The core kinase cascade is modulated by adaptor proteins, SAV1 (Salvador, also known as WW45) and MOB1 (encoded by MOB1A and MOB1B in human), both of which work to promote Hippo pathway signaling. MOB1 directly binds to LATS1 and LATS2, and additionally to two related kinases, NDR1, (gene name STK38) and NDR2 (gene name STK38L) via a specialized MOB1-binding domain N-terminal to the kinase domain (15; also see accompanying manuscript by Xiong et al., 2017). Key to its function as a Hippo pathway activator is the ability of MOB1 to bind directly to MST1 and MST2 kinases. We demonstrate that autophosphorylation of MST1 and MST2 on several threonine residues provides multiple MOB1 binding sites with varying binding affinities which in turn contribute to a redundancy of MST1-MOB1 protein interactions in cells.

Peptide overlay analysis (here referred to as Far-Western) revealed that peptides bearing phosphorylated forms of T353 and T367 consistently gave the highest binding signals across the array; nonphosphorylated versions of these peptides generated little to no binding signal. MST1 T353 and T367 peptides displayed high phospho-dependent binding affinities for MOB1A, with Kds of 280 nm and 680 nm for the phosphorylated peptides, respectively, and no detectable binding for the nonphosphorylated peptides. Consistent with their P0 positional binding preferences, human MOB1 bound more tightly to the MST1 pT367 peptide than to the optimized Nud1-like phosphoserine containing peptide than did yeast Mob1, and vice versa. The observed binding modes revealed by these structures are in close agreement with the binding modes reported previously for a yeast Nud1 derived phosphopeptide in complex with human MOB1A, as well as a MST2 T378 phosphopeptide in complex with human MOB1B (see ref 21, 22). As predicted by prior mutational data, the MST1 pT353 and pT367 phosphopeptides bound to the MOB1A phospho-binding pocket first identified by Rock et al., with the phosphate of the P0 threonine directly coordinated by K153, R154 and R157. The p + 1 side chains of M354 and M368 on MST1-pT353 and MST1-pT367 peptides respectively resided in an expansive hydrophobic surface composed by A89, A92, Y93, Y95, F156 and A160 side chains on MOB1A. The p + 3 side chain of I370 in the MST1-pT367 peptide oriented toward the same hydrophobic surface. The p + 2 side chains of I355 and V369 in MST1-pT353 and MST1-pT367 peptides respectively pointed to a distinct surface composed by M87, Y95 and the aliphatic portion of the E94 side chain on MOB1A. Thus, the hydrophobic nature of the p + 1 to p + 3 binding surfaces explained the consensus preferences for hydrophobic residues at these positions.

> MSFLFSSRSSKTFKPKKNIPEGSHQYELLKHAEATLGSGNLRQAVMLPEGEDLNEWIAVNTVDFFNQINMLYGTITEFCTEASCPVMSAGPRYEYHWADGTNIKKPIKCSAPKYIDYLMTWVQDQLDDETLFPSKIGVPFPKNFMSVAKTILKRLFRVYAHIYHQHFDSVMQLQEEAHLNTSFKHFIFFVQEFNLIDRRELAPLQELIEKLGSKDR;> DDTLPSQLGTMVINAED5-(4-bromophenyl)-7-phenyl-3,7-dihydro-4H-pyrrolo[2,3-d]pyrimidin-4-one | C18 H12 Br N3 O | 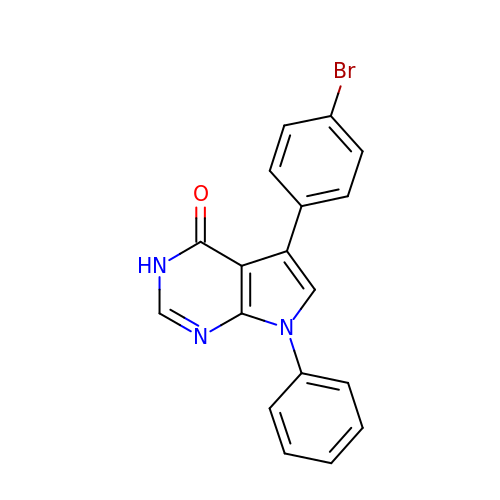CPYVKWBLVMVKFH-UHFFFAOYSA-N> MTWLSDFPQAWAETGGMGLAVRQAPLIIPLKATSTPVSIKQYPMSQEARLGIKPHIQRLLDQGILVPCQSPWNTPLLPVKKPGTNDYRPVQDLREVNKRVEDIHPTVPNPYNLLSGLPPSHQWYTVLDLKDAFFCLRLHPTSQPLFAFEWRDPEMGISGQLTWTRLPQGFKNSPTLFDEALH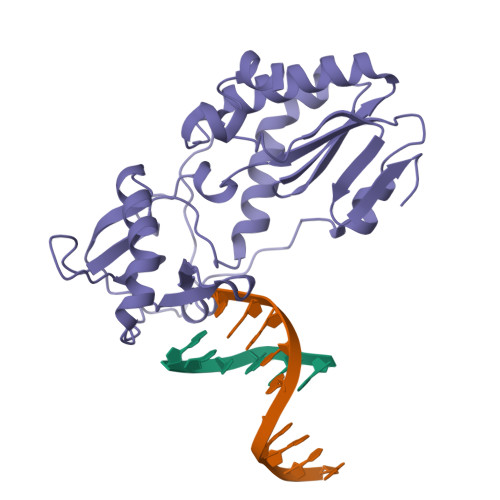RDLADFRIQHPDLILLQYVDDLLLAATSELDCQQGTRALLQTLGNLGYRASAKKAQICQKQVKYLGYLLKEGQR>MRIIMPVEFSRIVRDVERLIAVEKYSLQGVVDGDKLLVVGFSEGSVNAYLYDGGETVKLNREPINSVLDPHYGVGRVILVRDVSKGAEQHALFKVNTSRPGEEQRLEAVKPMRILSGVDTGEAVVFTGATEDRVALYALDGGGLRELARLPGFGFVSDIRGDLIAGLGFFGGGRVSLFTSNLSSGGLRVFDSGEGSFSSASISPGMKVTAGLETAREARLVTVDPRDGSVEDLELPSKDFSSYRPTAITWLGYLPDGRLAVVARREGRSAVFIDGERVEAPQGNHGRVVLWRGKLVTSHTSLSTPPRIVSLPSGEPLLEGGLPEDLRRSIAGSRLVWVESFDGSRVPTYVLESGRAPTPGPTVVLVHGGPFAEDSDSWDTFAASLAAAGFHVVMPNYRGSTGYGEEWRLKIIGDPCGGELE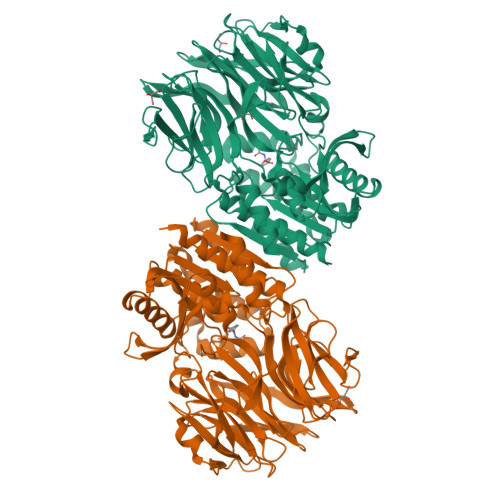DVSAAARWARESGLASELYIMGYSYGGYMTLCALTMKPGLFKAGVAGASVVDWEEMYELSDAAFRNFIEQLTGGSREIMRSRSPINHVDRIKEPLALIHPQNDSRTPLKPLLRLMGELLARGKTFEAHIIPDAGHAINTMEDAVKILLPAVFFLATQRERR[2x]>[2x]MEIFKYMEHQDYEQLVICQDKASGL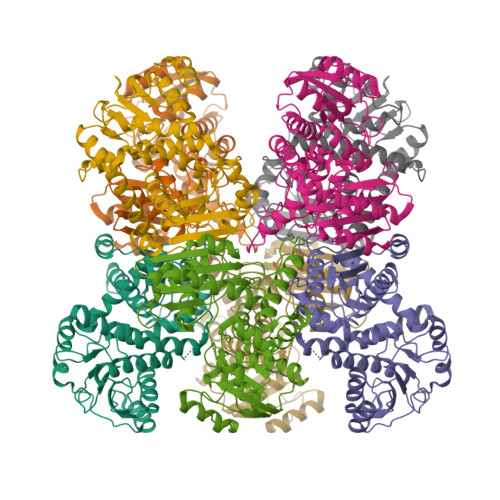KAIIAIHDTTLGPALGGTRMWTYASEEEAIEDALRLARGMTYKNAAAGLNLGGGKTVIIGNPKTDKNDEMFRAFGRYIEGLNGRYITAEDVGTTEADMDLINLETDYVTGTSAGAGSSGNPSPVTAYGIYYGMKAAAKEAFGDDSLAGKTVAVQGVGNVAYALCEYLHEEGAKLIITDINEEAVQRAVDAFGATAVGINEIYSQEADIFAPCALGAIINDETIPQLKAKVIAGSANNQLKETRHGDLIHEMGIVYAPDYVINSGGVINVADELDGYNRERALKRVEGIYDVIGKIFAISKRDNIPTYVAADRMAEERIARVANTRSTFLQNEKSVLSRR>SSDFVRKLYKMLEDPSYHSVVRWSDDGDSFVVLENEKFTKTILPKHFKHSNFASFVRQLNKYDFHKVRHNDENGESPYGRDAWEFKHPEFRADRKDNLDNIRRK[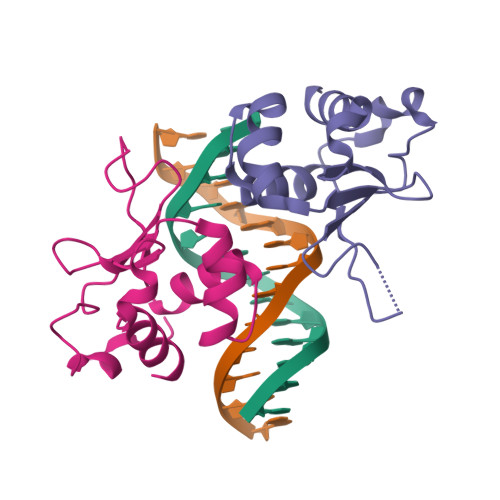2x]>MLKISTKGRYGLTIMIELAKKHGEGPTSLKSIAQTNNLSEHYLEQLVSPLRNAGLVKSIRGAYGGYVLGSEPDAITAGDIIRVL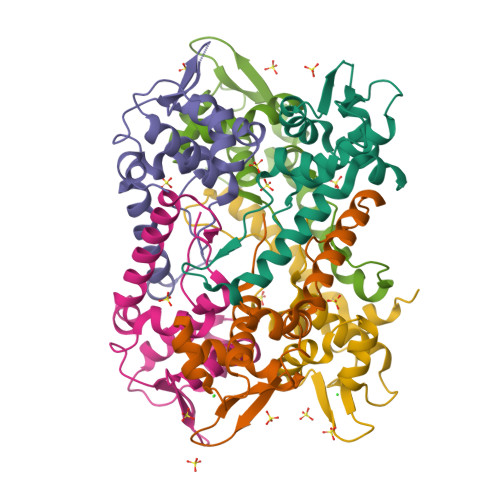EGPISPVEVLEDEEPAKRELWIRIRDAVKEVLDSTTLEDLASYTD[6x]>[2x]MSASHADQPTQTVSYPQLIDLLRRIFVVHGTSPEVADVLAENCASAQRDGSHSHGIFRIPGYLSSLASGWVDGKAVPVVEDVGAAFVRVDACNGFAQPALAAARSLLIDKARSAGVAILAIRGSHHFAALWPDVEPFAEQGLVALSMVNSMTCVVPHGARQPLFG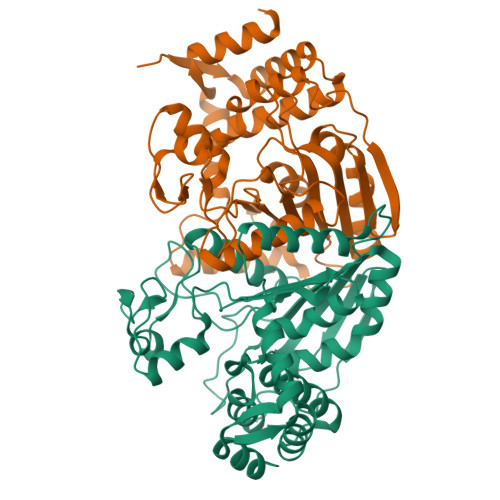TNPIAFGAPRAGGEPIVFDLATSAIAHGDVQIAAREGRLLPAGMGVDRDGLPTQEPRAILDGGALLPFGGHKGSALSMMVELLAAGLTGGNFSFEFDWSKHPGAQTPWTGQLLIVIDPDKGAGQHFAQRSEELVRQLHGVGQERLPGDRRYLERARSMAHGIVIAQADLERLQELAGH>MGHHHHHHHHSSGENLYFQGSKLEFMEGKTRTA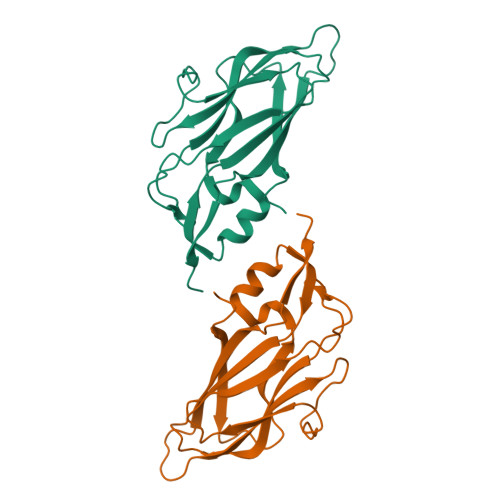PQGEAAGTATTASVPGTTTDGMDPGVVAATSVVTAENSSASVATAGIGGPPQQVDQQETWRTNFYYNDVFTWSVADAPGSILYTVQHSPQNNPFTAVLSQMYAGWAGGMQFRFIVAGSGVFGGRLVAAVIPPGIEIGPGLEVRQFPHVVIDARSLEPVTITMPDLRPNMYHPTGDPGLVPTLVLSVYNNLINPFGGSTNAIQVTVETRPSDDFEFVMIRAPS[2x]Mitochondrial transcription factor A (TFAM) plays a critical role in mitochondrial transcription initiation and mitochondrial DNA (mtDNA) packaging. Both functions require DNA binding, but in one case TFAM must recognize a specific promoter sequence, while packaging requires coating of mtDNA by association with non sequence-specific regions. TFAM is composed of two tandem high-mobility group (HMG) domains connected by an α-helix linker. In this study, we identified two TFAM residues, Ser61 in HMG box1 and Pro178 in HMG box2, that form specific hydrogen bonds with N2 of two guanine bases separated by 10 nucleotides (GN10G consensus).

Here, we have determined additional crystal structures of TFAM in complex with LSP (LSP_B) and a non-specific (NS2) DNA substrate. We were able to obtain data to 2.7 Å. Despite the shift, as in other crystal structures of TFAM-DNA substrates, in the TFAM-LSP_B structure, two HMG boxes interact tightly with the DNA duplex via the minor groove and generate two kink sites the intercalations of Leu58 (HMG box1) and Leu182 (HMG box2), inducing a U-turn in the DNA substrate. The α-helix linker connecting the two HMG boxes further enhances the binding of TFAM to the DNA duplex. Despite subtle differences in the sequence, the structure of TFAM-LSP_B revealed the same guanine-specific interactions as the other two TFAM-LSP structures, further highlighting the importance of these interactions and indicating that the TFAM binding site is not modulated by crystal packing. Replacement of both guanines in the expected guanine consensus to adenines (G-20/-31A(L), L stands for LSP) resulted in a ∼50% decrease in transcription activity. Thus, our results confirm that the G-20/-31(L) is important for proper transcriptional activity of TFAM. At the same time, the fact that eliminating the guanine pair does not completely eliminate initiation activity indicates that other factors must be involved in specific recognition of LSP by TFAM.

>SSVLASCPKKPVSSYLRFSKEQLPIFKAQNPDAKTTELIRRIAQRWRELPDSKKKIYQDAYRAEWQVYKEEISRFKEQLTPSQIMSLEKEIMDKHLKRKAMTKKKELTLLGKPKRPRSAYNVYVAERFQEAKGDSPQEKLKTVKENWKNLSDSEKELYIQHAKEDETRYHNEMKSWEEQMIEVGRKDLLRRTIKKQRKYGAEEC[2x]> MRALFYKDGKLFTDNNFLNPVSDNNPAYEVLQHVKIPTHLTDVVVYGQTWEEALTRLIFVGSDSKGRRQYFYGKMHVQNRNAKRDRIFVRVYNVMKRINSFINKNIKKSSTDSNYQLAVFMLMETMFFIRFGKMKYLKENETVGLLTLKNKHIEISPDKIVIKFVGKDKVSHEFVVHKSNRLYKPLLKLTDDSSPEEFLFNKL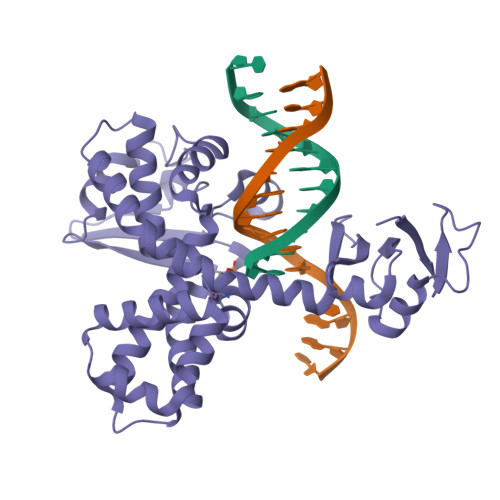SERKVYESIKQFGIRIKDLRTYGVNYTFLYNFWTNVKSISPLPSPKKLIALTIKQTAEVVGHTPSISKRAYMATTILEMVKDKNFLDVVSKTTFDEFLSIVVDHVKSSTDG> VEYRNWSKPQCQITGFAPFSKDNSIRLSAGGDIWVTREPYVSCDPVKCYQFALGQGTTLDNKHSNDTVHDRIPHRTLLMNELGVPFHLGTRQVCIAWSSSSCHDGKAWLHVCITGDDKNATASFIYDGRLVDSIGSWSQNILRTQESECVCINGTCTVVMTDGSASGRADTRILFIEEGKIVHISPLAGSAQHVEECSCYPRYPGVRCICRDNWKGSNRPVVDINMEDYSIDSSYVCSGLVGDTPRNDDRSSNSNCRNPNNERGTQGVKGWAFDNGNDLWMGRTISKDLRSGYETFKVIGGWSTPNSKSQINRQVIVDSDNRSGYSGIFSVEGKSCINRCFYVELIRGRKQETRVWW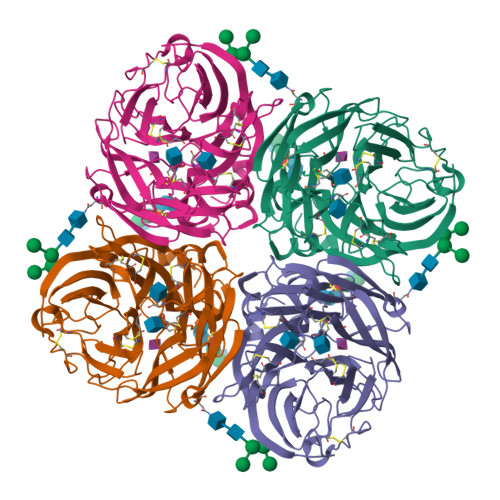TSNSIVVFCGTSGTYGTGSWPDGANINFMPI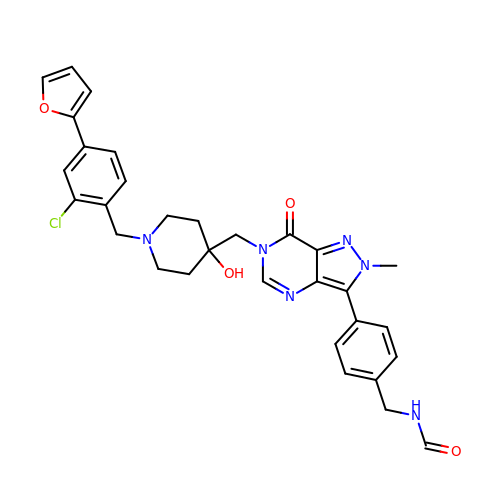~{N}-[[4-[6-[[1-[[2-chloranyl-4-(furan-2-yl)phenyl]methyl]-4-oxidanyl-piperidin-4-yl]methyl]-2-methyl-7-oxidanylidene-pyrazolo[4,3-d]pyrimidin-3-yl]phenyl]methyl]methanamide | C31 H31 Cl N6 O4 | NBSWPCOVWWWQAK-UHFFFAOYSA-N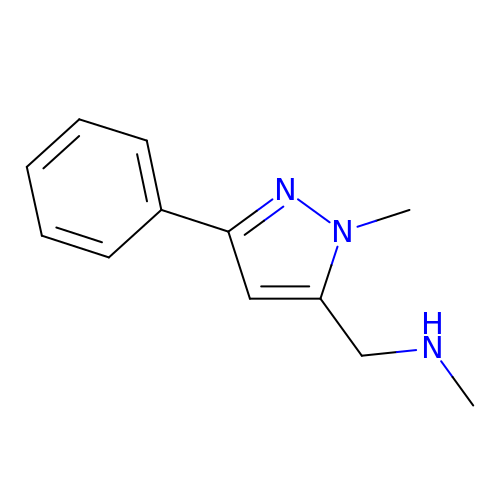methyl-3-methyl-5-phenyl-2H-pyrazol-4-methyl amine | C12 H15 N3 | QFUHILGXHQHXHY-UHFFFAOYSA-N> AMDVQETQKGALKEIQAFIRS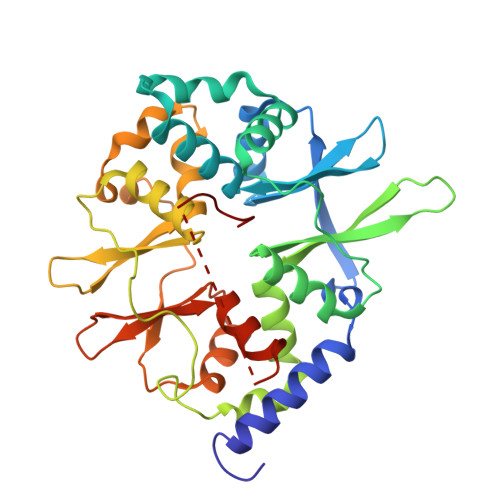RTSYDVLPTSFRLIVFDVTLFVKTSLSLLTLNNIVSAPLWDSEANKFAGLLTMADFVNVIKYYYQSSSFPEAIAEIDKFRLLGLREVERKIGAIPPETIYVHPMHSLMDACLAMSKSRARRIPLIDVDGETGSEMIVSVLTQYRILKFISMNCKETAMLRVPLNQMTIGTWSNLATASMETKVYDVIKMLAEKNISAVPIVNSEGTLLNVYESVDVMHLIQDGDYSNLDLSVGEALLKRPANFDGVHTCRATDRLDGIFDAIKHSRVHRLFVVDENLKLEGILSLADILNYIIYDKTTTPGVPEQTDNFESAV> MD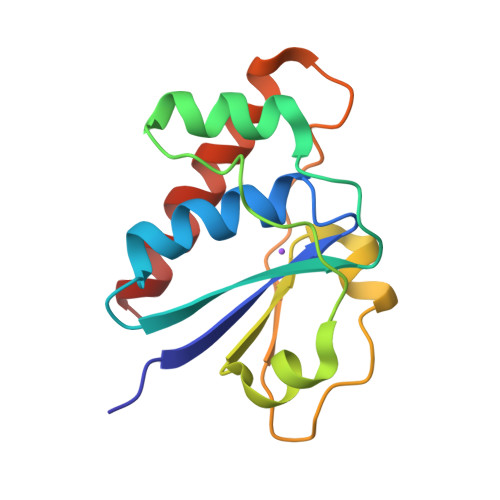KKTIYFICTGNSCRSQMAEGWGKEILGEGWNVYSAGIETHGVNPKAIEAMKEVDIDISNQTSDLIDNDILKQSDLVVTLCSDADNNCPILPPNVKKEHWGFDDPAGKEWSEFQRVRDEIKLAIEKFKLR> MNISDVAKITGLTSKAIRFYEEKGLVTPPMRS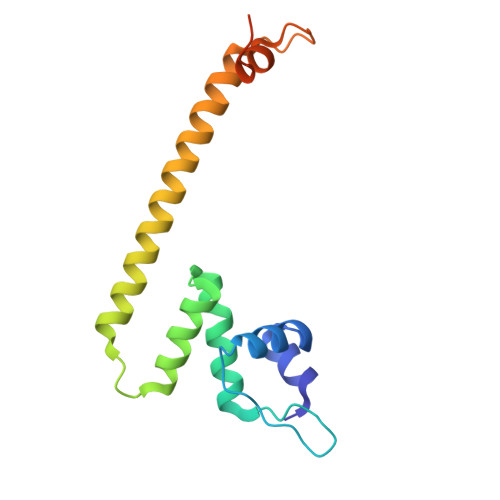ENGYRTYTQQHLNELTLLRQARQVGFNLEESGELVNLFNDPQRHSADVKRRTLEKVAEIERHIEELQSMRDQLLALANACPGDDSADCPIIENLSGCCHHRAGLEHHHHHH3-(4-fluorophenyl)benzoic 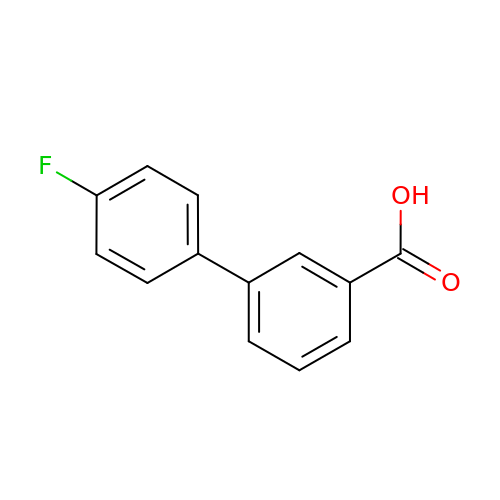acid | C13 H9 F O2 | YUQPLNXKGVRIAJ-UHFFFAOYSA-N>GMSEPQRLFFAIDLPAEIREQIIHWRAKHFPPEAGRPVAADNLHLTLAFLGEVSAEKEKALSLLAGRIRQPGFTLTLDDAGQWLRSRVVWLGMRQPPRGLIQLANMLRSQAARSGCFQSNRPFHPHITLLRDASEAVTIPPPGFNWSYAVTEFTLYASSFARGR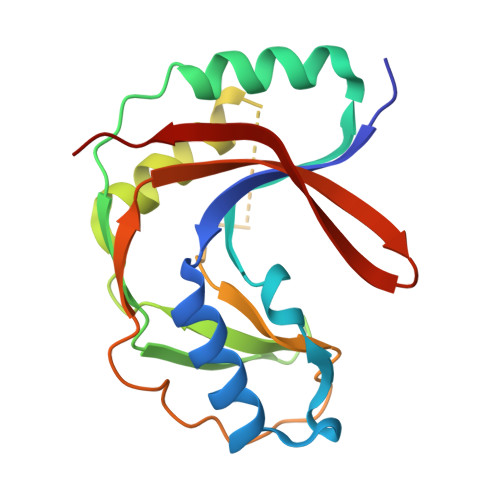TRYTPLKRWALTQ[2x]> GSHMGLTFNSNNICIDDNINTLWTGVNPTEANCQIMNSSESNDCKLILTLVKTGALVTAFVYVIGVSNNFNMLTTHRNINFTAELFFDSTGNLLTRLSSLKTPLNHKSGQNMATGAITNAKGFMPSTTAYPFNDNSREKENYIYGTCYYTASDRTAFPIDISVMLNRRAINDETSYCIRITW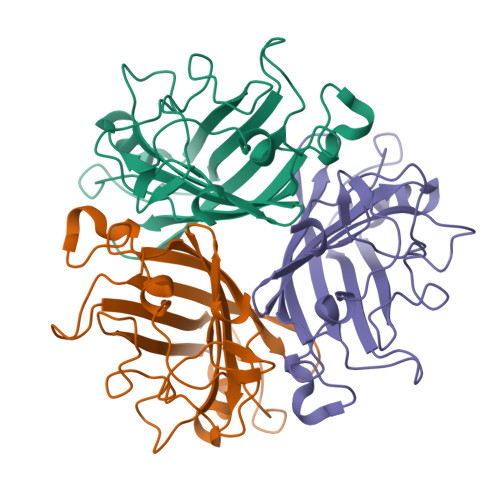SWNTGDAPEVQTSATTLVTSPFTFYYIREDD>HMTDLKASSLRALKLMDLTTLNDDDTDEKVIALCHQAKTPVGNTAAICIYPRFIPIARKTLKEQGTPEIRIATVTNFPHGNDDIDIALAETRAAIAYGADEVDVVFPYRALMAGNEQVGFDLVKACKEACAAANVLLKVIIET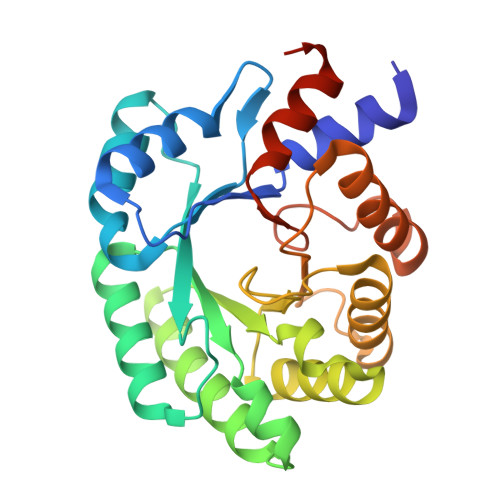GELKDEALIRKASEISIKAGADFIKTSTGKVAVNATPESARIMMEVIRDMGVEKTVGFKPAGGVRTAEDAQKYLAIADELFGADWADARHYRFGASSLLASLLKALGHGDGKSASSY[2x]>LSGAIVALILVIAGVIIAIAVVLFAFGLIPGISNQGSIQVLGSGTITNSTASGSSRTIYNITITVKNTGTTSISVTSININGQPFNINGTAPSIPAGRTQPITFEVTPASGKPNFSPGASYTATI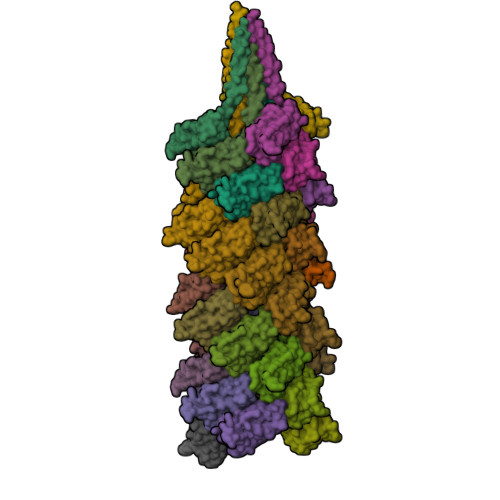YFSNGQGAPATLIYQG[37x]>[6x]MEFKKVAK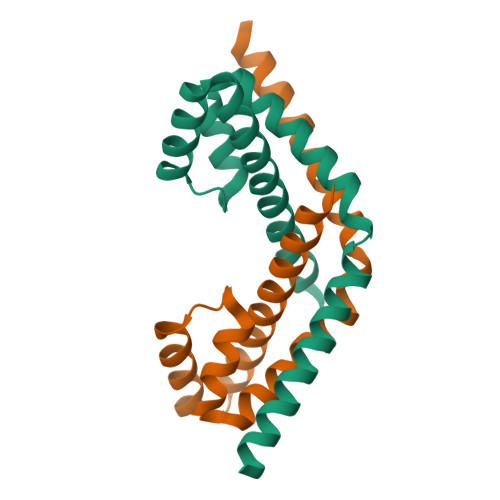ETAITLQSALTLQAVRLISQQLSETNPGQAIWLGEFSKRHPIQESDLYLEAMMLENKELVLRILTVRENLAEGVLEFLPEMVLSQIKQSNGNHRRSLLERLTQVDSSSTDQTEPNPGESDTSEDSE>MNFLRGVMGGQSAGPQHTEAETIQKLCDRVASSTLLDDRRNAVRALKSLSKKYRLEVGIQAMEHLIHVLQTDRSDSEIIGYALDTLYNIISNDEEEEVEENSTRQSEDLGSQFTEIFIKQQENVTLLLSLLEEFDFHVRWPGVKLLTSLLKQLGPQVQQIILVSPMGVSRLMDLLADSREVIRNDGVLLLQALTRSNGAIQKIVAFENAFERLLDIITEEGNSDGGIVVEDCLILLQNLLKNNNSNQNFFKEGSYIQRMKPWFEVGDENSGWSAQKVTNLHLMLQLVRVLVSPNNPPGATSSCQKAMFQCGLLQQLCTILMATGVPADILTETINTVSEVIRGCQVNQDYFASVNAPSNPPRPAIVVLLMSMVNERQPFVLRCAVLYCFQCFLYKNQKGQGEIVSTLLPSTIDATGNTVSAGQLLCGGLFSTDSLSNWCAAVALAHALQENATQKEQLLRVQLATSIGNPPVSLLQQCTNILSQGSKIQTRVGLLMLLCTWLSNCPIAVTHFLHNSANV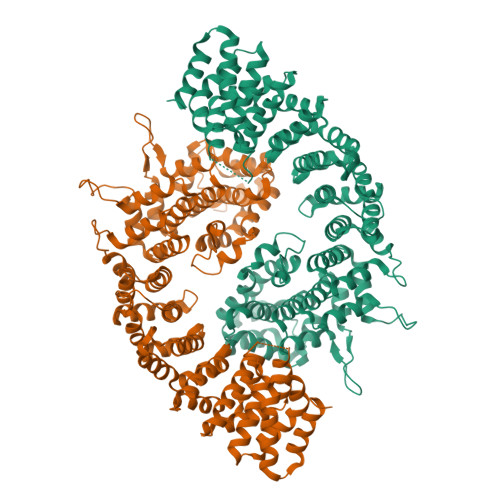PFLTGQIAENLGEEEQLVQGLCALLLGISIYFNDNSLETYMKEKLKQLIEKRIGKENFIEKLGFISKHELYSRASQKPQPNFPSPEYMIFDHEFTKLVKELEGVITKAIYKSSEEDKKEEEVKKTLEQHDSI[2x]> MSLKYGHVAWIQQILDGSYADAMNTLKNITVDDSKK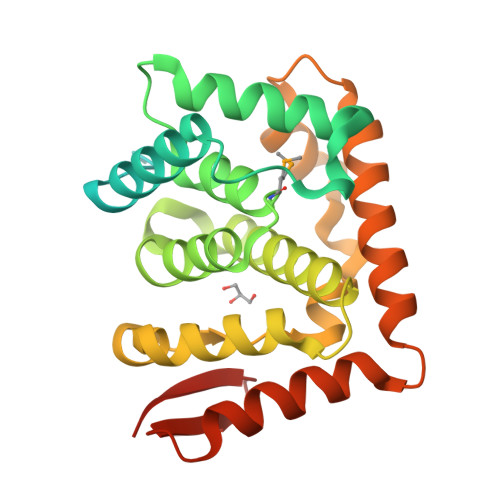GESLSECELHLNVAKLSSLLVEKDNLDINTLRKIQYNLDTIDAEKNISNKLKKGEVQICKRFKNGSIREVFNILVEELKSTTVVNLSDLVELYSMLDDEESLFIPLRLLSVDGNLLNFEVKKFLNALVWRRIVLLNASNEGDKLLQHIVKRVFDEELPKNNDFPLPSVDLLCDKSLLTPEYISETYGRFPIDQNAIREEIYEEISQVETLNSDNSLEIKLHSTIGSVAKEKNYTINYETNTVEYEGHHHHHH>[3x]MSNYPLHQACMENEFFKVQELLHSKPSLLLQKDQDGRIPLHWSVSFQAHEITSFLLSKMENVNLDDYPDDSGWTPFH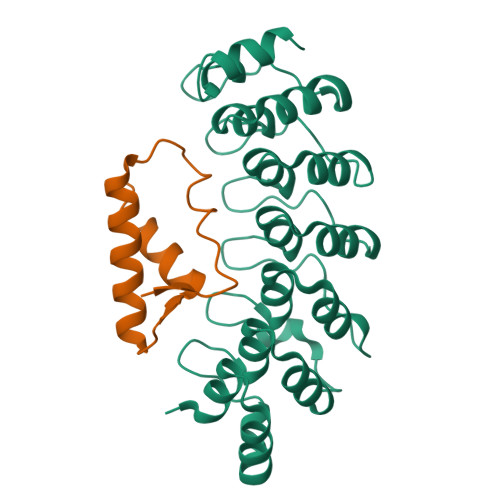IACSVGNLEVVKSLYDRPLKPDLNKITNQGVTCLHLAVGKKWFEVSQFLIENGASVRIKDKFNQIPLHRAASVGSLKLIELLCGLGKSAVNWQDKQGWTPLFHALAEGHGDAAVLLVEKYGAEYDLVDNKGAKAEDVALNEQVKKFFLNNV;>[3x]MERRLIFGTIASKMSLAPEADLDSLIIRNDSLSGAVIAAIMQEAGLRAVRKNRYVILQSDLEEAYATQVKTDNTVDKFDFYK> RLEILELLKNAAVRAGAQACFTCTLSEAVPVGEASWYIN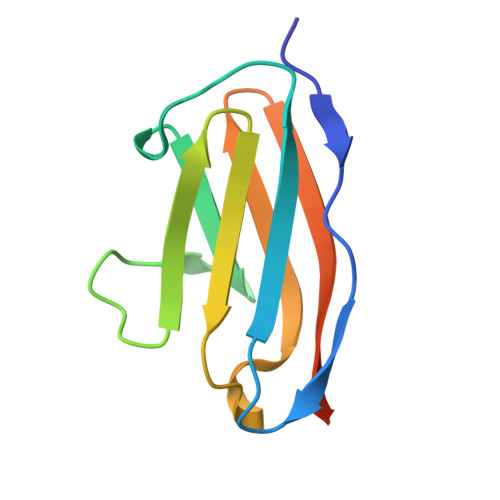GAAVQPDDSDWTVTADGSHHALLLRSAQPHHAGEVTFACRDAVASARLTVLGGLEHHHHHH> GDHPGLDALKDVLALPERPWRIEGYDNSNLFGTNIVSGMVVFEGGRSRRGEHRRFKVRGLEHPDDYESMKQTIYRRFTGSLADKLPLPDLMLIDGGRGQVNAALDALKEAGVQVPVVGLAKREERLILPGRYGAQWWLETGTEVGVDRELLLPHTH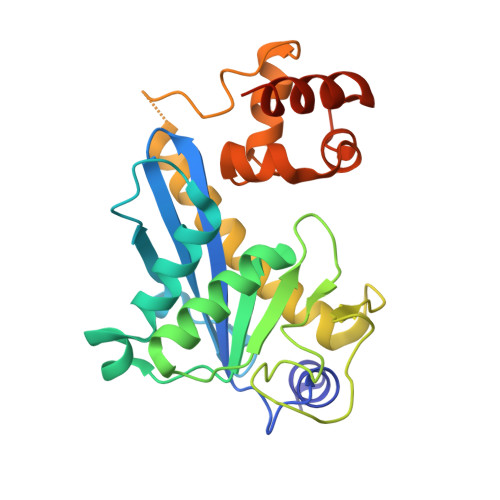PALRMLIGVRDEVHNYAVSYHRKLRGEGMLRSVFDDLPGIGQKRRDALLEHFTSLEDLAAAPVEHIAAVPGMTLRAAQSVKEFLQAREAQLPRAGG Cellular cargos move bidirectionally on microtubules by recruiting opposite polarity motors dynein and kinesin. Here we show that kinesin-3 KIF1C acts as both an activator and a processivity factor for dynein, using in vitro reconstitutions of human proteins. Unlike other cargo adapters, HOOKs form a stable assembly with two other accessory factors, FTS and FHIP. We provide a structural model for the autoinhibited FTS–HOOK3–FHIP1B (an FHF complex) and explain how KIF1C relieves it.

Our 3.2 Å reconstruction of full-length FTS and FHIP1B in complex with a C-terminal HOOK3 fragment (residues 571–718) allowed an atomic model to be built for each subunit. In the absence of HOOK3 the complex between FTS and FHIP1B does not form, suggesting that HOOK3 is central to FHF assembly. Our structure reveals HOOK3’s interactions involve the last of its four coiled-coil domains (CC4) and a C-terminal extension (CTE), consisting of a flexible region followed by a single alpha helix (residues 694–702). The first contact point (site 1) involves one of HOOK3’s two CTEs, with the helix latching onto a hydrophobic pocket within FHIP1B. Site 2 comprises a span of HOOK3 CC4 residues (653–688), packing tightly against the catalytically dead E2 ubiquitin ligase domain in FTS. At site 3, the opposite side of HOOK3 CC4 (spanning residues 663–670) binds a C-terminal alpha helix on FTS. This helix is situated within a long loop (FTS ‘belt’) that wraps around HOOK3 before docking into at the midzone of FHIP1B. Instead, the opposing face of FHIP1B comprises a highly conserved patch of surface-exposed residues. AlphaFold2 (AF) suggests this is a binding site for small G-protein Rab5, which has been shown to link FHF to early endosomes.

>DLEPRFNNSSLKIEELQEALRKKEEEMKQMEERYKKYLEKAKSVIRTLDPKQNQGAAPEIQALKNQLQERDRLFHSLEKEYEKTKSQREMEEKYIVSAWYNMGMTLHKKAAEDRLASTGSGQSFLARQRQATSSRRSYPGHVQPATAR[2x];> MERMNWLSRLASRGPGHRIPQGANLQTPVMADPETCLMVFKNHWSQVVRILERQGPRAAPGGADDLSAVRNHTYQMLTLLAEDRAVPSAPTGPGPLLEFALHEDLLTRVLTWQLQWDELGDGVEERRAEQLKLFEMLVSEARQPLLRHGPVREALLTLLDACGRPVPSSPALDEGLVLLLSQLCVCVAQEPSLLEFFLQPPPEPGAAPRLLLFSRLVPFVHLEGTLGQQARDALLLLMALSAGSPTVGRYIADHSYFCPVLATGLSALYSSLPRKIEVPGDDWHCLRREDWLGVPALALFMSSLEFCNAVIQVAHPLVQKQLVDYIHNGFLVPVMGPALHKTSVEEMIASTAYLELFLRSISEPALLRTFLRFLLLHRHDTHTILDTLVARIGSNSRLCMVSLSLFRTLLNLSCEDVLLQLVLRYLVPCNHVMLSQKPAVRDVDLYGRAADKFLSLIPRCCRHHAPSPPRPEHASWARGPGSPSVDSSSVTTVPRPSTPSRLALFLRQQSLGGSESPGPAPCSPGLSASPASSPGRRPTPAEEPGELEDNYLEYLREARRGVDRCVRACRTWSAPYDGERPSPEPSPFGSRTKKRSLLPEEDRNNVGEGEEEELGRRGRAGGAGEGPGHLPPPQLNGVPGSWPEGAKKVRLVPKEGAGELLEGISEGMAGLEGFGQELRELEVALSNGGTGSESPLEPPLPLEEEEAYESFTCPPEPPGPFLSSPLRTLNQLPSQPFTGPFMAVLFAKLENMLQNSVYVNFLLTGLVAQLACHPQPLLRSFLLNTNMVFQPSVKSLLQVLGSVKNKIENFAASQEDFPALLSKAKKYLIARGKLDWAEGPAAGPAPRRSDPLVKSRRPSLGELLLRHAHSPTRARQAAQLVLQPGRDGAGLGLSGGSPGASTPVLLTRGGAPERQGEALRVKNAVYCAVIFPEFLKELAAISQAHAVTSPFLLETSEEGSGPLISGCGPLNP;> MNPFWSMSTSSVRKRSEGEEKTLTGDVKTSPPRTAPKKQLPSIPKNALPITKPTSPAPAAQSTNGTHASYGPFYLEYSLLAEFTLVVKQKLPGVYVQPSYRSALMWFGVIFIRHGLYQDGVFKFTVYIPDNYPDGDCPRLVFDIPVFHPLVDPTSGELDVKRAFAKWRRNHNHIWQVLMYARRVFYKIDTASPLNPEAAVLYEKDIQLFKSKVVDSVKVCTARLFDQPKIEDPYAISFSPWNPSVHDEAREKMLTQKKPEEQHNKSVHVAGLSWVKPGSVQPFSKEEKTVAT>[5x]MTDMNILDLFLKASLLVKLIMLILIGFSIASWAIIIQRTRILNAAAREAEAFEDKFWSGIELSRLYQESQGKRDNLTGSEQIFYSGFKEFVRLHRANSHAPEAVVEGASRAMRISMNRELENLETHIPFLGTVGSISPYIGLFGTVWGIMHAFIALGAVKQATLQMVAPGIAEALIATAIGLFAAIPAVMAYNRLNQRVNKLELNYDNFMEEFTAILHRQAFTVSESNKG;>[2x]MARARGRGRRDLKSEINIVPLLDVLLVLLLIFMATAPIITQSVEVDLPDATESQAVSSNDNPPVIVEVSGIGQYTVVVEKDRLERLPPEQVVAEVSSRFKANPKTVFLIGGAKDVPYDEIIKALNLLHSAGVKSVGLMTQPI;>[3x]MSKATEQNDKLKRAIIISAVLHVILFAALIWSSFDENIEASAGGGGGSSIDAVMVDSGAVVEQYKRMQSQESSAKRSDEQRKMKEQQAAEELREKQAAEQERLKQLEKERLAAQEQKKQAEEAAKQAELKQKQAEEAAAKAAADAKAKAEADAKAAEEAAKKAAADAKKKAEAEAAKAAAEAQKKAEAAAAALKKKAEAAEAAAAEARKKAATEAAEKAKAEAEKKAAAEKAAADKKAAAEKAAADKKAAEKAAAEKAAADKKAAAEKAAADKKAAAAKAAAEKAAAAKAAAEADDIFGELSSGKNAPKTGGGAKGNNASPAGSGNTKNNGASGADINNYAGQIKSAIESKFYDASSYAGKTCTLRIKLAPDGMLLDIKPEGGDPALCQAALAAAKLAKIPKPPSQAVYEVFKNAPLDFKP

The Tol-Pal system is essential for maintaining outer membrane (OM) stability during cell division in Gram-negative bacteria. The inner membrane complex TolQRA harnesses proton motive force (PMF) to establish transient interactions within the periplasm, thereby coordinating cell envelope remodeling and facilitating OM invagination at division sites. TolQ forms a pentameric structure similar to that of MotA and ExbB, exhibiting a volcano-like configuration with a narrow periplasmic end and a wider cytoplasmic base. The pentameric TolQ encapsulates the dimeric TolR through its N-terminal transmembrane helices at the periplasmic end.

To address this, we co-expressed TolQR and TolA from Escherichia coli (strain K12), purified, and determined the structure of the TolQRA complex reconstituted in phospholipid nanodiscs by cryo-EM. The transmembrane portion of the complex, including TolQ and the transmembrane helices of TolR and TolA, is well resolved at 3.52 Å resolution. Densities for the periplasmic domains of TolA and TolR were obtained at lower resolution due to inherent flexibility. These regions were subsequently modeled through AlphaFold3 prediction. In the TolQRA nanodisc complex, we identified three major reconstructions showing up to three TolA molecules associated with TolQ subunits TolQ1, TolQ3, and TolQ4, respectively. TolA interacts with TolQ through their transmembrane helices (TolA_I) in a crossing configuration, stabilized by hydrogen bonds between TolQ_I29 and TolA_S18, TolQ_S28 and TolA_H22, and TolQ_N5 and TolA_S33. While D23 from TolR chain A (TolR(A)_D23) points toward the interface between TolQ2 and TolQ3, TolR(B)_D23 forms hydrogen bonds with T145 and T178 of TolQ5. When viewed from the cytoplasmic side of the pentamer, TolQ5R2A3 features an oval-shaped cytoplasmic opening, TolQ5R2 presents a round opening, and TolQ5R2A displays a split between TolQ1 and TolQ5 as well as between TolQ3 and TolQ4. In the cryo-EM map, we also observed a satellite periplasmic density located ~60 Å above TolQ5 and TolQ1, which likely corresponds to the periplasmic domains of TolR (TolR_PDs). A segment of this TolA1_loop is resolved in the cryo-EM map, protruding into the periplasmic space from the interface between helices 1 of TolQ1 and TolQ5, aligning with the TolR_PDs.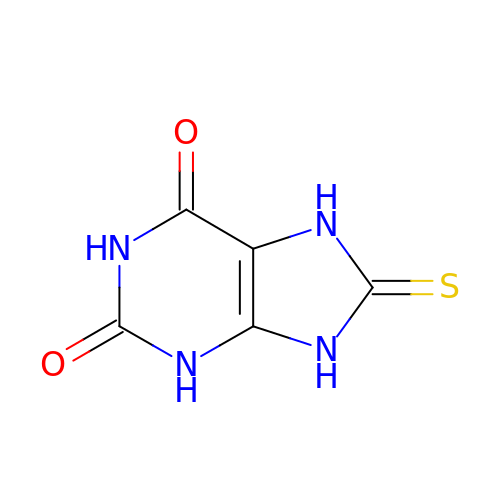8-thioxo-3,7,8,9-tetrahydro-1H-purine-2,6-dione | C5 H4 N4 O2 S | KFQXXACDWBTCDT-UHFFFAOYSA-N(3R)-3-({(4-aminobenzyl)[(4-aminophenyl)acetyl]amino}methyl)-5-{[(4-bromobenzoyl)oxy]methyl}-2,3,4,7-tetrahydro-1H-azepinium 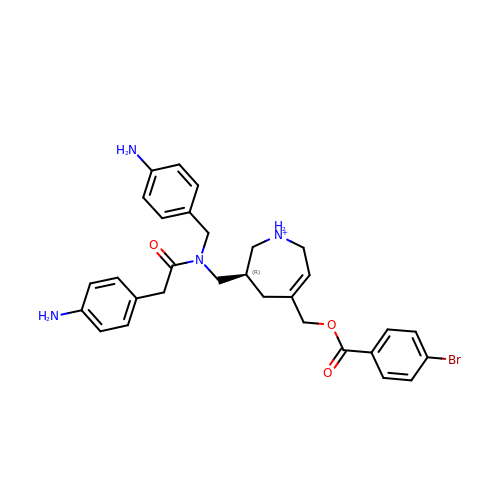| C30 H34 Br N4 O3 | ILVATMQGTNYMLQ-XMMPIXPASA-O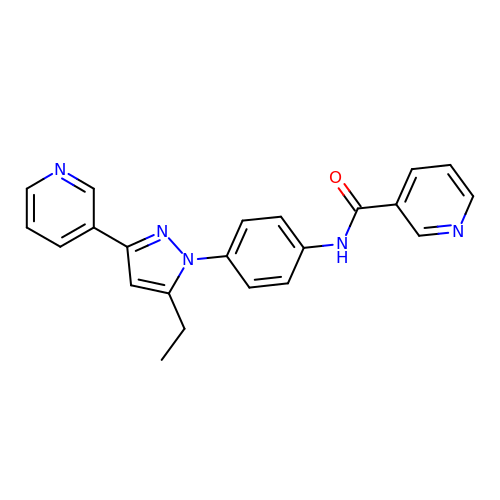N-[4-(5-ethyl-3-pyridin-3-yl-1H-pyrazol-1-yl)phenyl]pyridine-3-carboxamide | C22 H19 N5 O | CCAFHMPMIJBDRP-UHFFFAOYSA-N> AAQTNAPWGLARI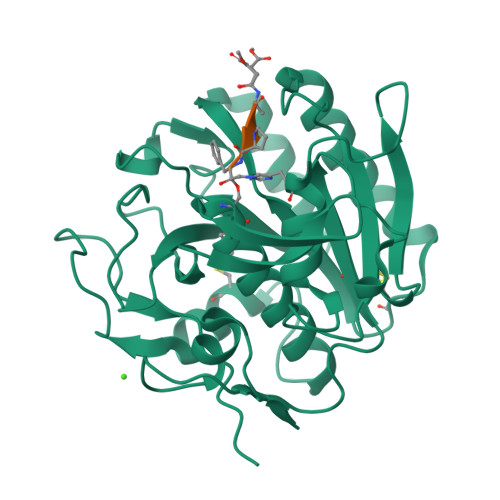SSTSPGTSTYYYDESAGQGSCVYVIDTGIEASHPEFEGRAQMVKTYYYSSRDGNGHGTHCAGTVGSRTYGVAKKTQLFGVKVLDDNGSGQYSTIIAGMDFVASDKNNRNCPKGVVASLSLGGGYSSSVNSAAARLQSSGVMVAVAAGNNNADARNYSPASEPSVCTVGASDRYDRRSSFSNYGSVLDIFGPGTDILSTWIGGSTRSISGTSMATPHVAGLAAYLMTLGKTTAASACRYIADTANKGDLSNIPFGTVNLLAYNNYQA;> XAAPF> HMSGPRKAPHFCPVCLRAFPYLSDLERHSISHSELKPHQCKVCGKTFKRSSHLRRHCNIHAGLRPFRCPLCPRRFREAGELAHHHRVHSGERPYQCPICRLRFTEANTLRRHAKRKHPEAMGVPLCAPDPGSEW

Here, we describe ZNF524, a zinc finger protein that directly binds telomeric repeats with nanomolar affinity, and reveal base-specific sequence recognition by cocrystallization with telomeric DNA. ZNF524 localizes to telomeres and specifically maintains the presence of the TRF2/RAP1 subcomplex at telomeres without affecting other shelterin members. Loss of ZNF524 concomitantly results in an increase in DNA damage signaling and recombination events. Overall, ZNF524 is a direct telomere-binding protein involved in the maintenance of telomere integrity.

To understand the interaction of the four zinc fingers with the telomeric motif in atomic detail, we crystallized the ZNF524 DNA-binding domain (107-237 aa) with telomeric DNA and solved its structure to 2.40 Å. In the crystal, each crystallographic asymmetric unit contained one ZNF524 minimal domain bound to a telomeric duplex DNA. The DNA molecules in the crystal are coaxially stacked, with the terminal A and T bases of neighboring DNA molecules pairing to form a pseudo continuous TTAGGG duplex. Each ZF adopts a canonical C2H2 zinc finger fold with its recognition α-helices inserted into the major groove, making base-specific contacts through both hydrogen bonds and van der Waals interactions. In agreement with the DNA pull-down and ITC results, all four ZFs form direct, base-specific interactions with telomeric DNA. In particular, ZF2 is central to the DNA interaction with the four amino acids Arg153, Ser155, His156 and Arg159, making base-specific contacts along a 4-bp region. Similarly, in ZNF524 ZF2, Arg159 donates two hydrogen bonds to the O6 and N7 atoms of G9, forming a bidentate H-bond interaction. Additionally, the Nε2 group of His156 donates one H-bond to the N7 atom of G10. However, Arg153 forms a van der Waals contact with the methyl group of T11, deviating from the ZBTB48 structure, where it recognizes the GGG triplet. Here, the RxxHxxR motif of ZF2 recognizes a TGG triplet instead of GGG, while the GGG triplet is jointly recognized by ZF2, ZF3 and ZF4.>[4x]SNAMEALKRKIEEEGVVLSDQVLKVDSFLNHQIDPLLMQRIGDEFASRFAKDGITKIVTIE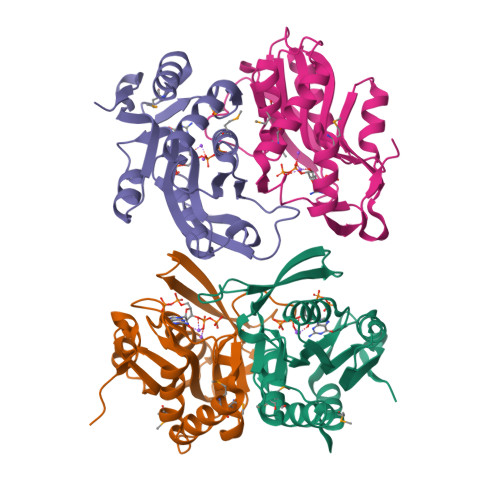SSGIAPAVMTGLKLGVPVVFARKHKSLTLTDNLLTASVYSFTKQTESQIAVSGTHLSDQDHVLIIDDFLANGQAAHGLVSIVKQAGASIAGIGIVIEKSFQPGRDELVKLGYRVESLARIQSLEEGKVSFVQEVHS> MDGTAAEPRPGAGSLQHAQPPPQPRKKRPEDFKFGKILGEGSFSTVVLARELATSREYAIKILEKRHIIKENKVPYVTRERDVMSRLDHPFFVKLYFTFQDDEKLYFGLSYAKNGELLKYIRKIGSFDETCTRFYTAEIVSALEYLHGKGIIHRDLKPENILLNEDMHIQITDFGTAKVLSPESKQARANAFVGTAQYVSPELLTEKSACKSSDLWALGCIIYQLVAGLPPFRAGNEYLIFQKIIKLEYDFPEKFFPK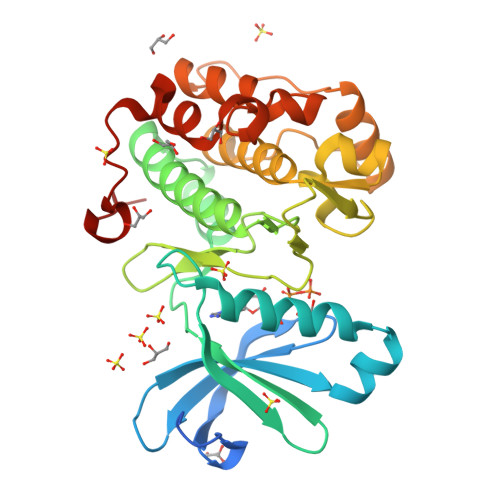ARDLVEKLLVLDATKRLGCEEMEGYGPLKAHPFFESVTWENLHQQTPPKLTA In Escherichia coli, cytotoxic DNA methyl lesions on the N1 position of purines and N3 position of pyrimidines are primarily repaired by the 2-oxoglutarate (2-OG) iron(II) dependent dioxygenase, AlkB. AlkB is a member of the iron(II) dependent 2-oxoglutarate (2-OG) dioxygenase superfamily that couples decarboxylation of 2-OG to succinate to oxidation of methylation damage primarily in the form of 1-methyladenine (1-meA) and 3-methylcytosine (3-meC) upon binding of dioxygen to the iron(II) cofactor. The AlkB enzyme recognizes and repairs other alkylated DNA lesions such as 3-methylthymine (3-meT), 1-methylguanine (1-meG), and 1,N6-ethenoadenine (εA), albeit with lower efficiency. AlkB repairs methylated DNA damage in ssDNA much more efficiently than in duplex DNA and displays significantly different activity on structurally similar methylated bases.

Here we present the structures of the full length E. coli D135A AlkB in complex with ssDNA containing a 1-meG lesion and the unliganded wild-type AlkB holoenzyme. We determined the structure of the full length E. coli AlkB protein in complex with a 17-mer ssDNA oligonucleotide containing a 1-meG lesion to 2.2 Å resolution and the structure of the AlkB holoenzyme in the absence of nucleotide substrate to 2.9 Å resolution. The protein was crystallized under aerobic conditions in complex with 2-OG and cobalt(II) as the metal ion. The use of cobalt supports DNA binding but prevents catalytic activity. Greater insight into DNA binding and substrate base recognition comes from a comparison of the AlkB-ssDNA complex with the AlkB holoenzyme structure. The hydroxyl side chain of T51 is positioned to make hydrogen bonding interactions with the backbone amide nitrogen of residue Y55 to stabilize the conformation of the T51-Y55 loop. Superposition of our structures of the AlkB-ssDNA complex with the unliganded AlkB proteins (core r.m.s.d = 0.772 Å) reveals little difference structurally in the global conformation of the proteins. Instead, our data indicate that AlkB is a fairly rigid molecule, and the flexibility and dynamics of the nucleotide recognition lid is more localized to residues Y76 and the T51-Y55 loop and not the whole domain, although we cannot rule out movement of this domain during intermediate DNA binding steps. Our comparison of nucleic acid bound and unliganded structures reveals that residue Y76 undergoes a conformational change upon DNA binding necessary for damaged bases to bind in the active site and subsequent catalysis.

>GPHMLDLFADAEPWQEPLAAGAVILRRFAFNAAEQLIRDINDVASQSPFRQMVTPGGYTMSVAMTNCGHLGWTTHRQGYLYSPIDPQTNKPWPAMPQSFHNLCQRAATAAGYPDFQPDACLINRYAPGAKLSLHQDKDEPDLRAPIVSVSLGLPAIFQFGGLKRNDPLKRLLLEHGDVVVWGGESRLFYHGIQPLKAGFHPLTIDCRYNLTFRQAGKKE[2x]> VGGYTEPRSVTPEERSVFQPMILSKLLTAGSVVSSCELELLQVSTQVVAGTNY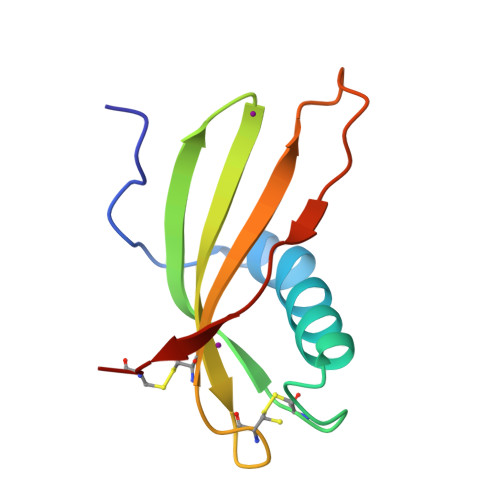KFKVSGGATCPGCWEVVVFVPLYSSKSATSVGTPTRVSCT(1R,2S,3R,1S',1S")Phosphoric acid mono(4-{2-[1-(1,2-dicarbamoylethylcarbamoyl)-3-carbamoylpropylcarbamoyl]-3-methylcarbamoylcyclopropyl}phenyl) 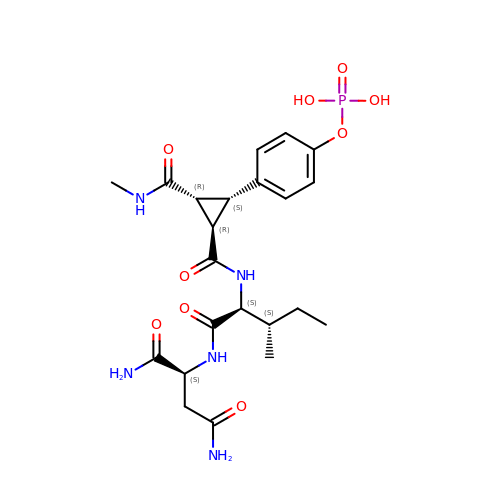ester | C22 H32 N5 O9 P | TXAWBRUKEBJWOA-LWVFFRLXSA-N>MASTVSNTSKLEKPVSLIWGCELNEQNKTFEFKVEDDEEKCEHQLALRTVCLGDKAKDEFHIVEIVTQEEGAEKSVPIATLKPSILPMATMVGIELTPPVT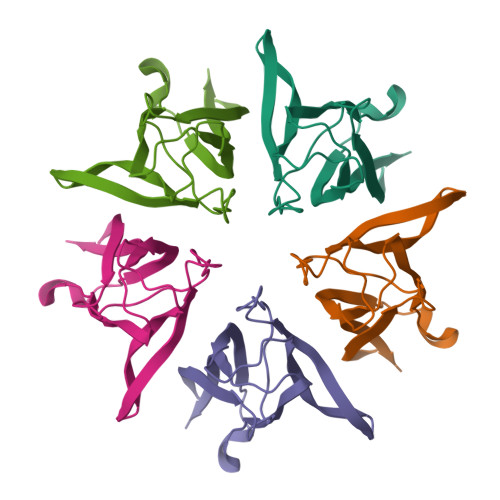FRLKAGSGPLYISGQHVAMEEDYSWAEEEDEGEAEGEEEEEEEEDQESPPKAVKRPAATKKAGQAKKKLDKEDESSEEDSPTKKGKGAGRGRKPAAKK[5x]> MPGSAAKGSELSERIESFVETLKRGGGPRSSEEMARETLGLLRQIITDHRWSNAGELMELIRREGRRMTAAQPSETTVGNMVRRVLKIIREEYGRLHGRSDESDQQESLHKLLTSGGLNEDFSFHYAQLQSNIIEAINELLVELEGTMENIAAQALEHIHSNEVIMTIGFSRTVEAFLKEAARKRKFHVIVAECAPFCQGHEMAVNLSKAGIETTVMTDAAIFA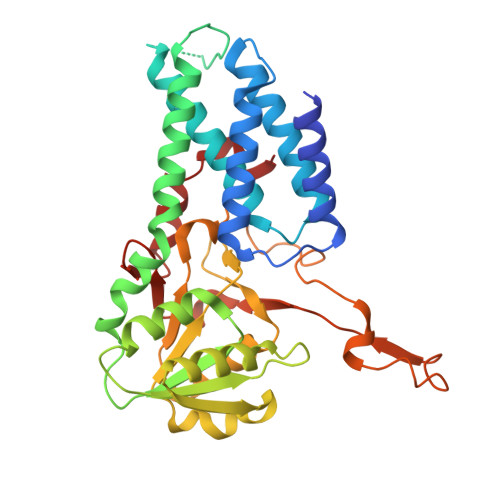VMSRVNKVIIGTKTILANGALRAVTGTHTLALAAKHHSTPLIVCAPMFKLSPQFPNEEDSFHKFVAPEEVLPFTEGDILEKVSVHCPVFDYVPPELITLFISNIGGNAPSYIYRLMSELYHPDDHVL ORF3a is a transmembrane protein capable of forming homodimers and potentially homotetramers. The TRAF proteins participate in multiple NF-κB signaling pathways, functioning as adaptor proteins and E3 ubiquitin ligases. They form trimers and interact with receptor intracellular domains and other proteins through their C-terminal TRAF-C domains. Since the putative TRAF-binding sequence in ORF3a is conserved between SARS-CoV (PLQAS) and SARS-CoV-2 (PIQAS), and generally conforms to the TRAF-binding consensus sequences, we hypothesized that SARS-CoV-2 ORF3a might also bind to TRAFs and thereby induce NF-κB activation.

To investigate whether the SARS-CoV-2 ORF3a N-terminal region containing the PIQAS sequence is capable of binding to TRAF molecules, we crystallized the TRAF2 TRAF-C domain and the TRAF3 TRAF-C domain in complex with a 16-amino acid peptide from the N-terminal region of ORF3a (residues 30–45). The crystallographic asymmetric unit in the TRAF2 crystal lattice contains three TRAF-C molecules forming a trimer, while the asymmetric unit in the TRAF3 crystal lattice contains six TRAF-C molecules forming two trimers. We observed density for five residues (PIQAS) of the ORF3a peptide, which binds at a solvent-facing groove in the globular region of the TRAF-C domain. The TRAF-C binding sites are not fully occupied—in our model, each TRAF trimer has either one or two peptides bound, which is similar to previously reported TRAF:peptide complex structures. The ORF3a peptide forms several main chain and side chain hydrogen bonds with the surrounding residues from TRAF2 or TRAF3. Of note, the side chain from Q38 in the peptide forms multiple hydrogen bonds with two serine residues in the TRAF-C domain. The S40 side chain is also within hydrogen bonding distance of TRAF residues that may contribute to peptide binding. Additionally, the P36 residue, also highly conserved among TRAF2/3-binding peptides, is in proximity to other hydrophobic and aromatic residues in the TRAF molecule, particularly F511, with which it may form hydrophobic interactions. The binding affinities between the PIQAS peptide and SUMO-TRAF-C proteins were in the range of 150–200 μM (192.5 μM for TRAF2 and 171.6 μM for TRAF3). Crystal structures revealed that a PIQAS-containing peptide can bind to TRAF2 or TRAF3 at the previously identified peptide-binding surface in the TRAF-C domain.

>NTGLLESQLSRHDQMLSVHDIRLADMDLRFQVLETASYNGVLIWKIRDYKRRKQEAVMGKTLSLYSQPFYTGYFGYKMCARVYLNGDGMGKGTHLSLFFVIMRGEYDALLPWPFKQKVTLMLMDQGSSRRHLGDAFKPDPNSSSFKKPTGEMNIASGCPVFVAQTVLENGTYIKDDTIFIKVIVDTSDLPDP[6x];>[3x]PIQAS>[7x]MADSDINIKTGTTDIGSNTTVKTGDLVTYDKENGMHKKVFYSFIDDKNHNKKLLVIRTKGTIAGQYRVYSEEGANKSGLAWPSAFKVQLQLPDNEVAQISDYYPRNSIDTKEYFSTLTYGFNGNVTGDDTGKIGGLIGANVSIGHTLKYVQPDFKTILESPTDKKVGWKVIFNNMVNQNW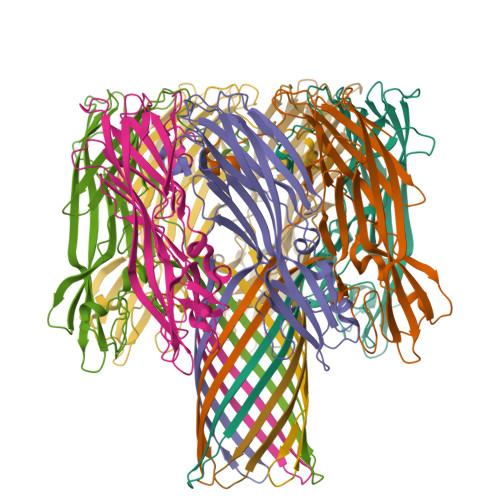GPYDRDSWNPVYGNQLFMKTRNGSMKAADNFLDPNKASSLLSSGFSPDFATVITMDRKASKQQTNIDVIYERVRDDYQLHWTSTNWKGTNTKDKWTDRSSERYKIDWEKEEMTN>MNVGDNSNFFVIKAKENGVNVFGMTRGTDTRFHHSEKLDKGEVMIAQFTEHTSAVKIRGKAIIQTSYGTLDTE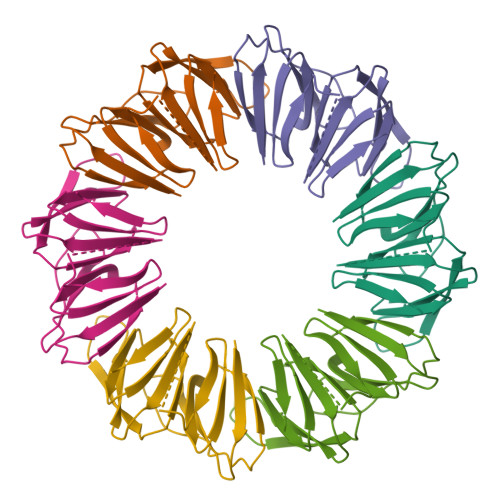KDEGGGGSGGGGSMNVGDNSNFFVIKAKENGVNVFGMTRGTDTRFHHSEKLDKGEVMIAQFTEHTSAVKIRGKAIIQTSYGTLDTEKDEENLYFQ[6x]> MRHISPEELIALHDANISRYGGLPGMSDPGRAEAIIGRVQARVAYEEITDLFEVSATYLVATARGHIFND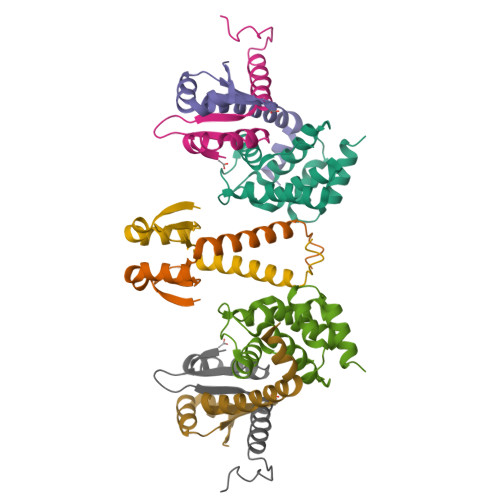ANKRTALNSALLFLRRNGVQVFDSPELADLTVGAATGEISVSSVADTLRRLYGSAE;>[3x]MQSINFRTARGNLSEVLNNVEAGEEVEITRRGREPAVIVSKATFEAYKKAALDAEFASLFDTLDSTNKELVNR> SEFRRQTIRHSTREKDRGPTKATTTKLVYQIFDTFFAEQIEKDDREDKENAFKRRRCGVCEVCQQPECGKCKACKDMVKFGGSGRSKQACQERRCPNMAMKEADDDEEVDDNIPEMPSPKKMHQGKKKKQNKNRISWVGEAVKTDGKKSYYKKVCIDAETLEVGDCVSVIPDDSSKPLYLARVTALWEDSSNGQMFHAHWFCAGTDTVLGATSDPLELFLVDECEDMQLSYIHSKVKVIYKAPSENWAMEGGMDPESLLEGDDGKTYFYQLWYDQDYARFESPPKTQPTEDNKFKFCVSCARLAEMRQKEIPRVLEQLEDLDSRVLYYSATKNGILYRVGDGVYLPPEAFTFNIKLSSPVKRPRKEPVDEDLYPEHYRKYSDYIKGSNLDAPEPYRIGRIKEIFCPKKSNGRPNETDIKIRVNKFYRPENTHKSTPASYHADINLLYWSDEEAVVDFKAVQGRCTVEYGEDLPECVQVYSMGGPNRFYFLEAYNAKSKS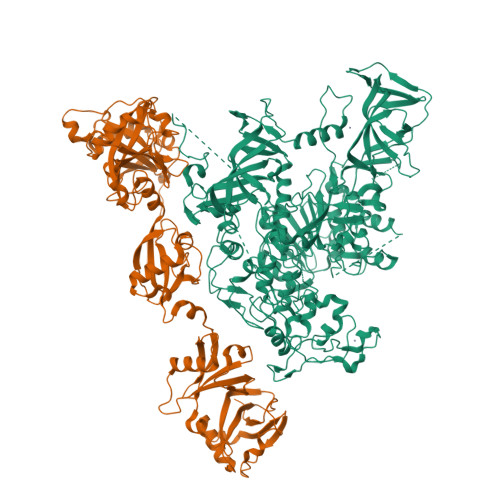FEDPPNHARSPGNKGKGKGKGKGKPKSQACEPSEPEIEIKLPKLRTLDVFSGCGGLSEGFHQAGISDTLWAIEMWDPAAQAFRLNNPGSTVFTEDCNILLKLVMAGETTNSRGQRLPQKGDVEMLCGGPPCQGFSGMNRFNSRTYSKFKNSLVVSFLSYCDYYRPRFFLLENVRNFVSFKRSMVLKLTLRCLVRMGYQCTFGVLQAGQYGVAQTRRRAIILAAAPGEKLPLFPEPLHVFAPRACQLSVVVDDKKFVSNITRLSSGPFRTITVRDTMSDLPEVRNGASALEISYNGEPQSWFQRQLRGAQYQPILRDHICKDMSALVAARMRHIPLAPGSDWRDLPNIEVRLSDGTMARKLRYTHHDRKNGRSSSGALRGVCSCVEAGKACDPAARQFNTLIPWCLPHTGNRHNHWAGLYGRLEWDGFFSTTVTNPEPMGKQGRVLHPEQHRVVSVRECARSQGFPDTYRLFGNILDKHRQVGNAVPPPLAKAIGLEIKLCMLAKA;> GPLGSEAHLYMQVQIVAEDQFCGHQGNDMYDEEKVKYTVFKVLKNSSLAEFVQSLSQTMGFPQDQIRLWPMQARSNGTKRPAMLDNEADGNKTMIELSDNENPWTIFLETVDPELAASGATLPKFDKDHDVMLFLKMYDPKTRSLNYCGHIYTPISCKIRDLLPVMCDRAGFIQDTSLILYEEVKPNLTERIQDYDVSLDKALDELMDGDIIVFQKDDPENDNSELPTAKEYFRDLYHRVDVIFCDKTIPNDPGFVVTLSNRMNYFQVAKTVAQRLNTDPMLLQFFKSQGYRDGPGNPLRHNYEGTLRDLLQFFKPRQPKKLYYQQLKMKITDFENRRSFKCIWLNSQFREEEITLYPDKHGCVRDLLEECKKAVELGEKASGKLRLLEIVSYKIIGVHQEDELLECLSPATSRTFRIEEIPLDQVDIDKENEMLVTVAHFHKEVFGTFGIPFLLRIHQGEHFREVMKRIQSLLDIQEKEFEKFKFAIVMMGRHQYINEDEYEVNLKDFEPQPGNMSHPRPWLGLDHFNKAPKRSRYTYLEKAIKIHN(~{N}~{Z})-~{N}-[(5~{S})-4-ethanoyl-5-methyl-5-phenyl-1,3,4-thiadiazolidin-2-ylidene]ethanamide 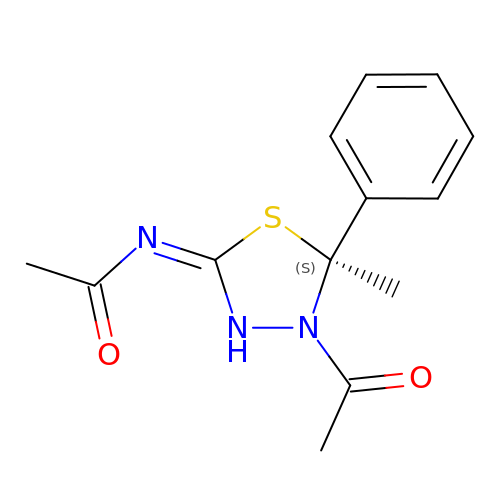| C13 H15 N3 O2 S | JEFVYQYZCAVNTP-ZDUSSCGKSA-N1-[(3R)-3-[(3R,4R,5S,6R,7R,8S,9S,10R,13R,14S,17R)-6-ethyl-4-fluoranyl-10,13-dimethyl-3,7-bis(oxidanyl)-2,3,4,5,6,7,8,9,11,12,14,15,16,17-tetradecahydro-1H-cyclopenta[a]phenanthren-17-yl]butyl]-3-(phenylsulfonyl)urea 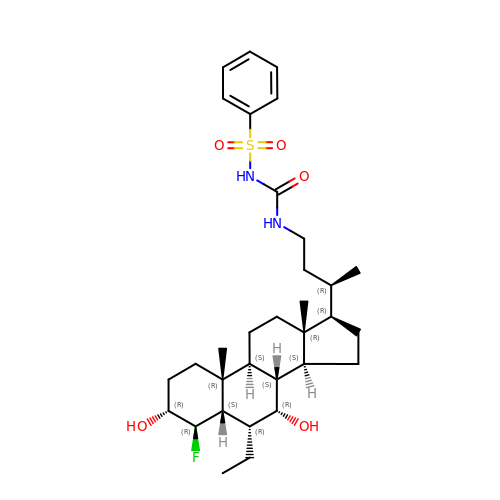| C32 H49 F N2 O5 S | QVNPKOJFMSHZPJ-PTJGPXMYSA-N(2~{S},3~{R})-3-methyl-2-[(2~{S},3~{R})-3-oxidanyl-1-oxidanylidene-butan-2-yl]-4-[(3~{S},5~{S})-5-[(sulfamoylamino)methyl]pyrrolidin-3-yl]sulfanyl-3,4-dihydro-2~{H}-pyrrole-5-carboxylic acid | C15 H26 N4 O6 S2 | 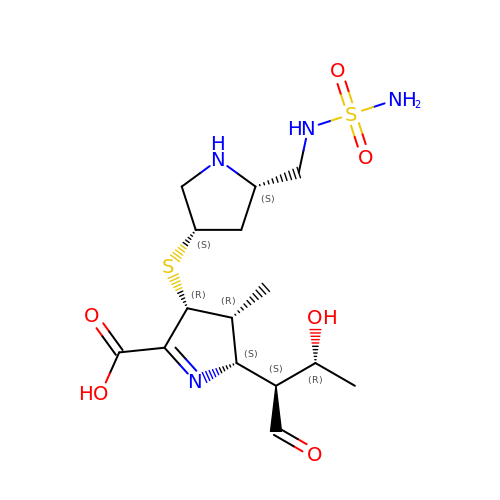RBKUPZPTQNSPAV-QZOCKBNKSA-N> AFVVTDNCIKCKYTDCVEVSPVDCFYEGPNFLVIHPDECIDCALCEPECPAQAI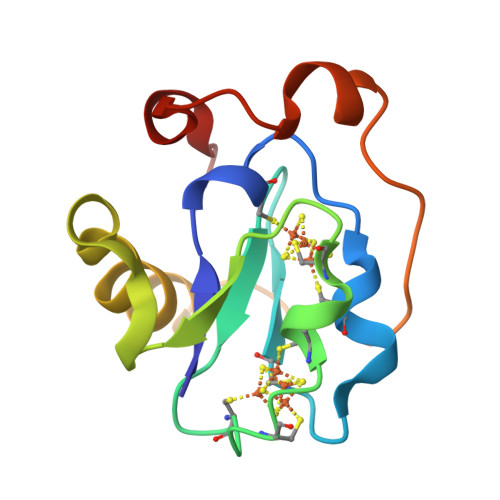FSEDEVPEDMQEFIQLNAELAEVWPNITEKKDPLPDAEDWDGVKGKLQHLER> MSSTHIEQFMPVKLAQALANSLFPELDSQLRAGRHIGIDDLDNHAFLMDFQEQLEEFYARYNVELIRAPEGFFYLRPRSTTLIPRSVLSELDMMVGKILCYLYLSPERLANQGIFTSQELYEELISLADEG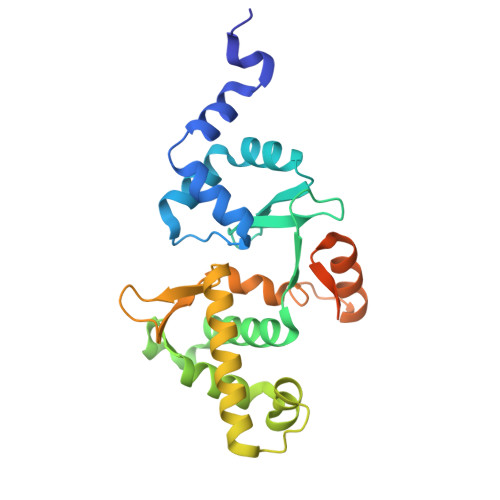KLMKFVNQRSSGSDLDKQKLQEKVRTTLNRLRRLGMVYFLPNNNNKFTITEAVFRFGADVRSGDDPREIQLRMIRDGEAMPVEGSLSLDDSENDETPDNSAEGAGDEQP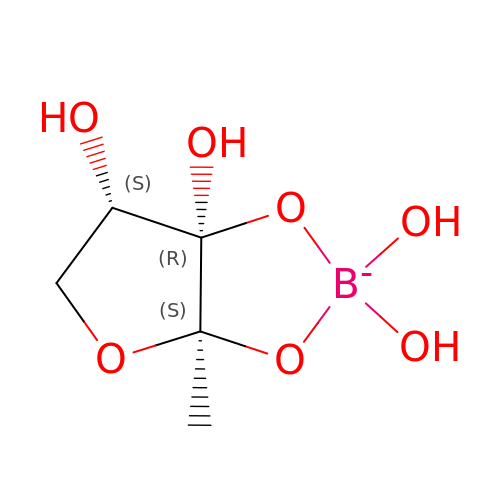3A-METHYL-5,6-DIHYDRO-FURO[2,3-D][1,3,2]DIOXABOROLE-2,2,6,6A-TETRAOL | C5 H10 B O7 | ACKRRKSNOOISSG-VPENINKCSA-N> MLKQVEIFTDGSALGN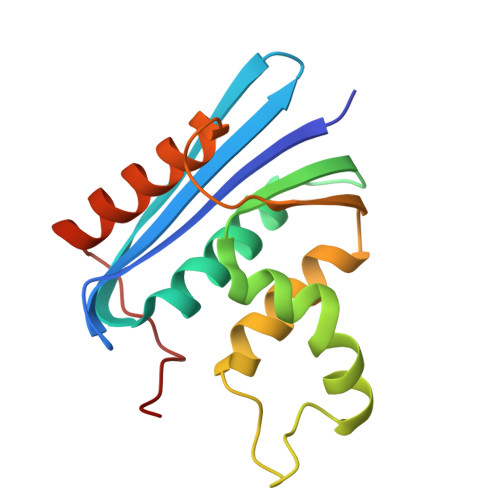PGPGGYGAILRYRGREKTFSAGYTRTTNNRMELMAAAVALEALKEHAEVILSTDSQYVRQGITQWIHNWKKRGWKTADKKPVKNVDLWQRLDAALGQHQIKWEWVKGHAGHPENERADELARAAAMNPTLEDTGYQVEV The l-type amino acid transporters (LATs) mediate neutral amino acids and thyroid hormones across membrane. LAT1 or LAT2 are the light chains of the heterodimeric amino acid transporters (HATs), which are composed of a light chain and a heavy chain. LAT2, which is mainly expressed in kidney and small intestine, has a broader substrate range than LAT1, including small amino acids. Here, we report the cryo-EM structures of the human LAT2–4F2hc complex bound with substrate Leu or Trp at resolution of 2.9 or 3.4 Å, respectively.

The cryo-EM structures of the LAT2–4F2hc complex incubated with Leu or Trp were determined at 2.9 and 3.4 Å resolution, respectively. The cryo EM maps of LAT2–4F2hc + Leu and LAT2–4F2hc + Trp are very similar to each other. The overall structure of LAT2–4F2hc revealed an inward-open conformation, with Leu or Trp substrate binding to the bottom of the inner pocket of LAT2. Interestingly, the Trp substrate shows a triangular star-shaped density in the map, into which we assigned two binding positions for Trp. In position 1, Trp exhibits similar binding mode to Leu, while in position 2, the α-amino and α-carboxylate group of Trp mainly interact with the TM3 and TM10 in LAT2, forming hydrogen bonds with Asn134 in TM3 and Asn395 in TM10, respectively. To validate the binding modes, we introduced the N134Q, F243A, and N395Q mutants in LAT2 and set up the counterflow assay. Results showed that the F243A mutation had almost no transport activity. The N134Q and N395Q mutations remained ~20% transport activity compared with wild type (WT) in the [14C]-Trp and Leu counterflow assay, or remained ~15% and ~40% transport activity in the [3H]-Leu and Leu counterflow assay, respectively, suggesting their important roles in the transport cycle of LAT2. We propose that the Asn134-binding and Asn395-binding state might represent an intermediate state of substrate recognition and transport during an alternating assess cycle. Actually, the corresponding residues for Asn134 and Asn395 in LAT2 are Ser and Asn in LAT1 and ASC1, which are capable to form hydrogen bonds with substrates, suggesting the putative dual-binding-mode described here might also exist in LAT1 and ASC1.

> MAHHHHHHHHHHSGRELQPPEASIAVVSIPRQLPGSHSEAGVQGLSAGDDSETGSDCVTQAGLQLLASSDPPALASKNAEVTVETGFHHVSQADIEFLTSIDPTASASGSAGITGTMSQDTEVDMKEVELNELEPEKQPMNAASGAAMSLAGAEKNGLVKIKVAEDEAEAAAAAKFTGLSKEELLKVAGSPGWVRTRWALLLLFWLGWLGMLAGAVVIIVRAPRCRELPAQKWWHTGALYRIGDLQAFQGHGAGNLAGLKGRLDYLSSLKVKGLVLGPIHKNQKDDVAQTDLLQIDPNFGSKEDFDSLLQSAKKKSIRVILDLTPNYRGENSWFSTQVDTVATKVKDALEFWLQAGVDGFQVRDIENLKDASSFLAEWQNITKGFSEDRLLIAGTNSSDLQQILSLLESNKDLLLTSSYLSDSGSTGEHTKSLVTQYLNATGNRWCSWSLSQARLLTSFLPAQLLRLYQLMLFTLPGTPVFSYGDEIGLDAAALPGQPMEAPVMLWDESSFPDIPGAVSANMTVKGQSEDPGSLLSLFRRLSDQRSKERSLLHGDFHAFSAGPGLFSYIRHWDQNERFLVVLNFGDVGLSAGLQASDLPASASLPAKADLLLSTQPGREEGSPLELERLKLEPHEGLLLRFPYAALE;> MADYKDDDDKSGPDEVDASGREEGARHRNNTEKKHPGGGESDASPEAGSGGGGVALKKEIGLVSACGIIVGNIIGSGIFVSPKGVLENAGSVGLALIVWIVTGFITVVGALCYAELGVTIPKSGGDYSYVKDIFGGLAGFLRLWIAVLVIYPTNQAVIALTFSNYVLQPLFPTCFPPESGLRLLAAICLLLLTWVNCSSVRWATRVQDIFTAGKLLALALIIIMGIVQICKGEYFWLEPKNAFENFQEPDIGLVALAFLQGSFAYGGWNFLNYVTEELVDPYKNLPRAIFISIPLVTFVYVFANVAYVTAMSPQELLASNAVAVTFGEKLLGVMAWIMPISVALSTFGGVNGSLFTSSRLFFAGAREGHLPSVLAMIHVKRCTPIPALLFTCISTLLMLVTSDMYTLINYVGFINYLFYGVTVAGQIVLRWKKPDIPRPIKINLLFPIIYLLFWAFLLVFSLWSEPVVCGIGLAIMLTGVPVYFLGVYWQHKPKCFSDFIELLTLVSQKMCVVVYPEVERGSGTEEANEDMEEQQQPMYQPTPTKDKDVAGQPQP>[2x]MSLGNIFVTGRIAFSLKYEQQTQSLVVHVKECHQLAYADEAKKRSNPYVKTYLLPDKSRQGKRK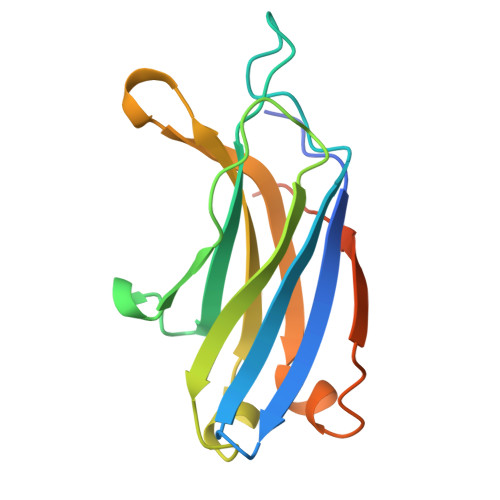TSIKRDTVNPLYDETLRYEIPESLLAQRTLQFSVWHHGRFGRNTFLGEAEIQMDSWKLDKKLDHCLPLHGKISAESEGHHHHHH>[2x]SYYHHHHHHLESTSLYKKAGLQRTLVLIKPDAFERSLVAEIMGRIEKKNFKIVSMKFWSKAPRNLIEQHYKEHSEQSYFNDNCDFMVSGPIISIVYE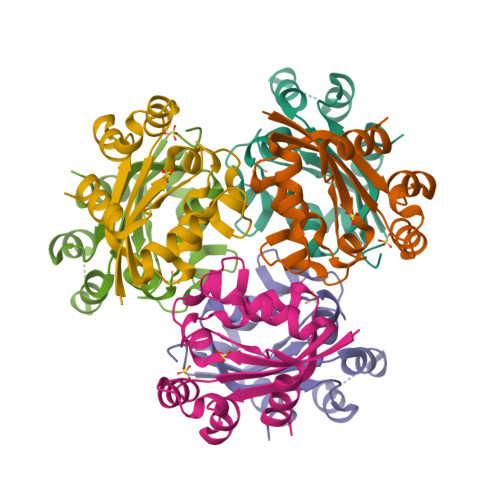GTDAISKIRRLQGNILTPGTIRGDLANDIRENLIHASDSEDSAVDEISIWFPETKMETDN>[3x]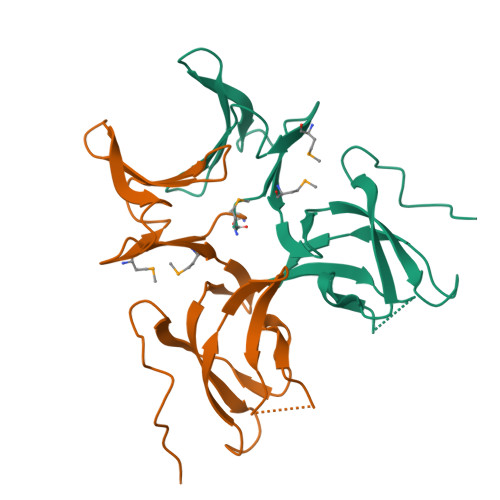MNTAYRVWDGEQMHYWDDEGLSLIIKSNGDWTLKRLYTDVLVPVVDSTNRNAALMWGAKVRGKFIYDRSIVKITSDDKESSDVCEVKFSDGVFQVDVSKISADYDVTAVGWVEYATIEVIGDVYQNPELLEGVKLEHHHHHH> IVGGYTCAANSIPYQVSLNS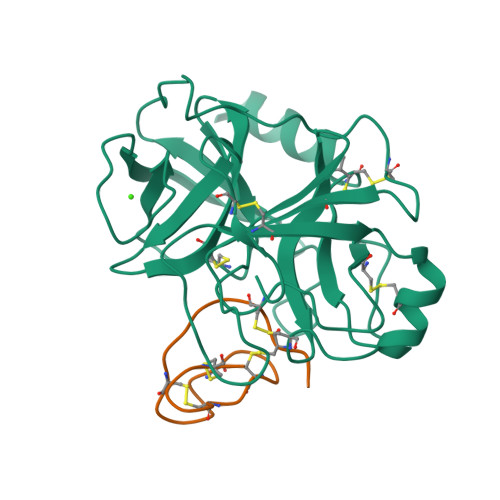GSHFCGGSLINSQWVVSAAHCYKSRIQVRLGEHNIDVLEGNEQFINAAKIITHPNFNGNTLDNDIMLIKLSSPATLNSRVATVSLPRSCAAAGTECLISGWGNTKSSGSSYPSLLQCLKAPVLSNSSCKSSYPGQITGNMICVGFLQGGKDSCQGDSGGPVVCNGQLQGIVSWGYGCAQKNKPGVYTKVCNYVNWIQQTIAAN;> RICPRIWMECTRDSDCMAKCICVAGHCG>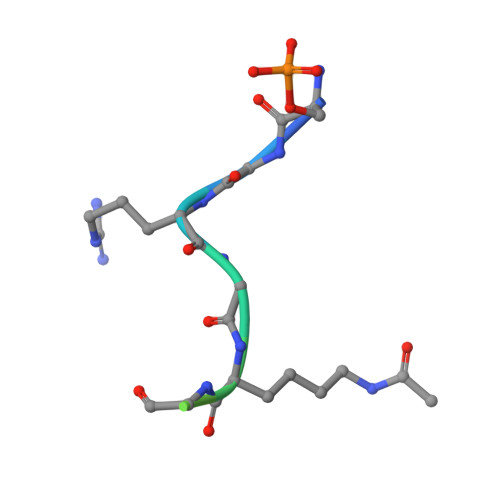 SGRGKGGKGLGKGG> GPSGTSHMLTLARQQQRQNIRWLLSLSVLMLLALLLSLSAGEQWISPGDWFTPRGELFVWQIRLPRTLAVLLVGAALAISGAVMQALFENPLAEPGLLGVSNGAGVGLIAAVLLGQGQLPNWALGLSAIAGALIITLILLRFARRHLSTSRL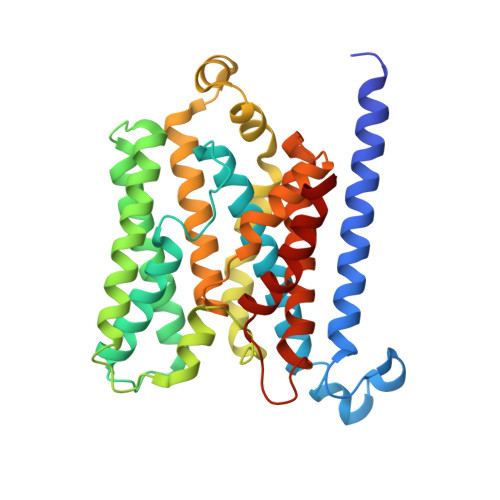LLAGVALGIISSALMTWAIYFSTSVDLRQLMYWMMGGFGGVDWRQSWLMLALIPVLLWISSQSRPMNMLALGEISARQLGLPLWFWRNVLVAATGWMVGVSVALAGAIGFIGLVIPHILRLSGLTDHRVLLPGCALAGASALLLADIVARLALAAAELPIGVVTATLGAPVFIWLLLKAGR[(2~{R},3~{S},4~{S},5~{R})-5-(6-aminopurin-9-yl)-3,4-bis(oxidanyl)oxolan-2-yl]methoxy-~{N}-[2-(1~{H}-indol-3-yl)ethyl]phosphonamidic acid | C20 H24 N7 O6 P | 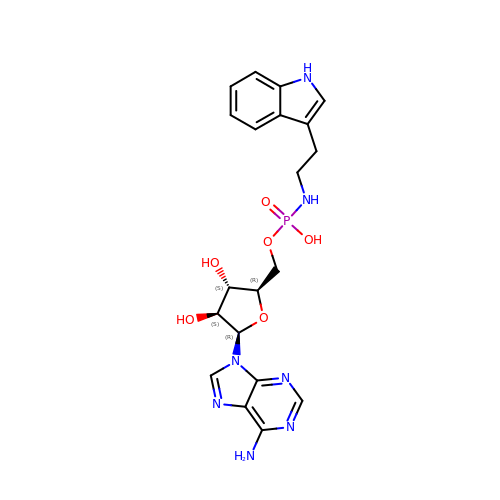QUYHGTZYKXLUHM-DFYYWFRZSA-N>[12x]ISEFGSTMARAIYDFFSTP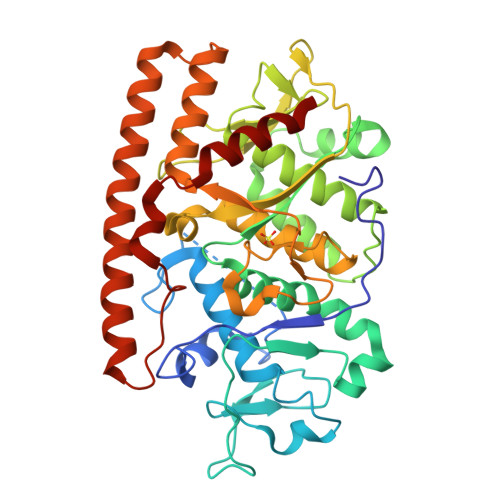FGNRGLATNRTQLSSLLSSSNSPWQRFLSSMTPLTAPGIVSTPEAPYPGSLMYQESMLHSATVPGVLGSRDAWRTFNVFGLSWTDEGLSGLVAAQDPPPAAPYQPASAQWSDLLNYPRWANRRRELQSKYPLLLRSTLLSAMRAGPVLYVETWPNMISGRLADWFMSQYGNNFVDMCARLTQSCSNMPVEPDGNYDQQMRALISLWLLSYIGVVNQTNTISGFYFSSKTRGQALDSWTLFYTTNTNRVQITQRHFAYVCARSPDWNVDKSWIAAANLTAIVMACRQPPVFANQGVINQAQNRPGFSMNGGTPVHELNLLTTAQECIRQWVMAGLVSAAKGQALTQEANDFSNLIQADLGQIKAQDDALYNQQPGYARRIKPFVNGDWTPGMTAQALAVLATFTA> GLEEKKENKQLTYTTVKDIGDMNPHVYGGSMSAESMIYEPLVRNTKDGIKPLLAKKWDVSEDGKTYTFHLRDDVKFHDGTPFDADAVKKNIDAVQENKKLHSWLKISTLIDNVKVKDKYTVELNLKEAYQPALAELAMPRPYVFVSPKDFKNGTTKDGVKKFDGTGPFKLGEHKKDESADFNKNDQYWGEKSKLNKVQAKVMPAGETAFLSMKKGETNFAFTDDRGTDSLDKDSLKQLKDTGDYQVKRSQPMNTKMLVVNSGKKDNAVSDKTVRQAIGHMVNRDKIAKEILDGQEKPATQLFAKNVTDINFDMPTRKYDLKKAESLLDEAGWKKGKDSDVRQKDGKNLEMAMYYDKGSSSQKEQAEYLQAEFKKMGIKLNINGETSDKIAERRTSGDYDLMFNQTWGLLYDPQSTIAAFKAKNGYESATSGIENKDKIYNSIDDAFKIQNGKERSDAYKNILKQIDDEGIFIPISHGSMTVVAPKDLEKVSFTQSQYELPFN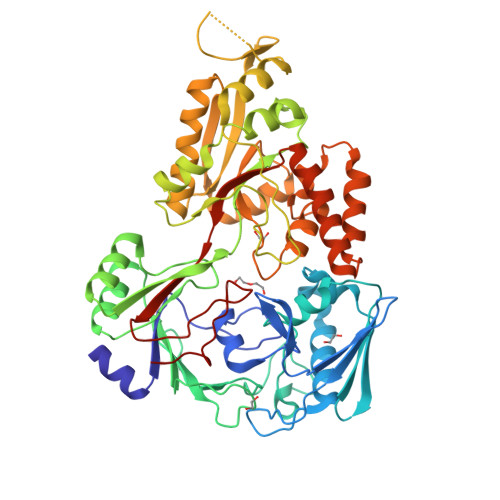EMQYK> SVDHGFLVTRHSQTIDDPQCPSGTKILYHGYSLLYVQGNERAHGQDLGTA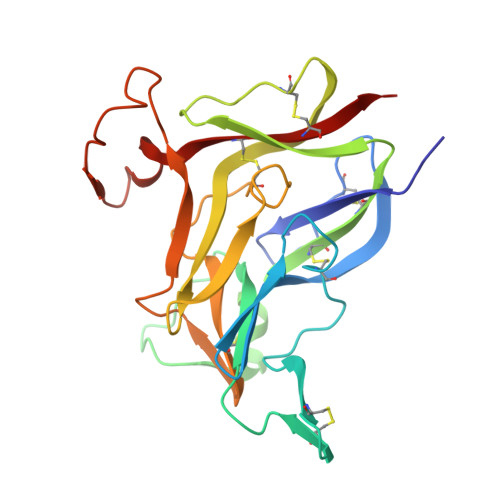GSCLRKFSTMPFLFCNINNVCNFASRNDYSYWLSTPEPMPMSMAPITGENIRPFISRCAVCEAPAMVMAVHSQTIQIPPCPSGWSSLWIGYSFVMHTSAGAEGSGQALASPGSCLEEFRSAPFIECHGRGTCNYYANAYSFWLATIERSEMFKKPTPSTLKAGELRTHVSRCQVCMRRT2-[3,6-bis(oxidanyl)-9~{H}-xanthen-9-yl]-5-[(6-oxidanyl-6-oxidanylidene-hexyl)carbamothioylamino]benzoic 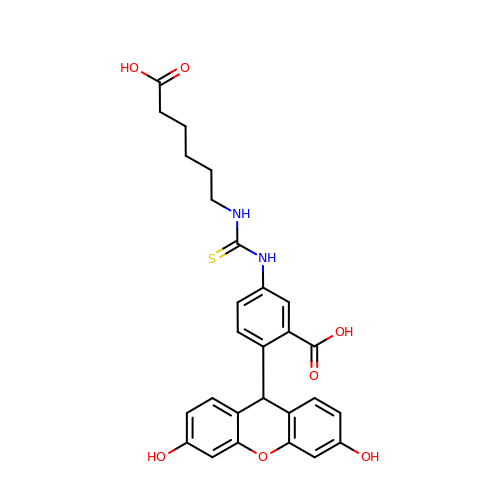acid | C27 H26 N2 O7 S | RDYFZBSVNLLBMW-UHFFFAOYSA-N>ASVHGTTYELLRRQGIDTVFGNPGSNELPFLKDFPEDFRYILALQEACVVGIADGYAQASRKPAFINLHSAAGTGNAMGALSNAWNSHSPLIVTAGQQTRAMIGVEALLTNVDAANLPRPLVKWSYEPASAAEVPHAMSRAIHMASMAPQGPVYLSVPYDDWDKDADPQSHHLFDRHVSSSVRLNDQDLDILVKALNSASNPAIVLGPDVDAANANADCVMLAERLKAPVWVAPSAPRCPFPTRHPCFRGLMPAGIAAISQLLEGHDVVLVIGAPVFRYHQYDPGQYLKPGTRLISVTCDPLEAARAPMGDA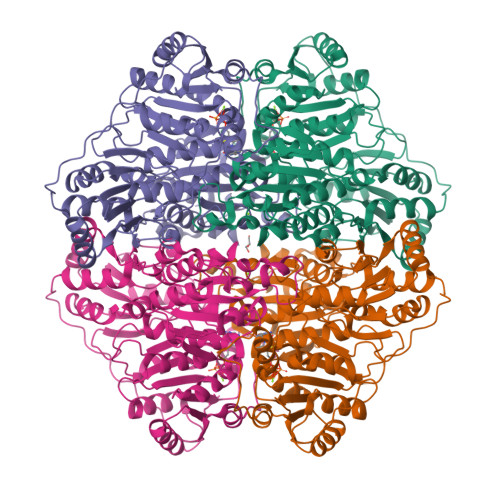IVADIGAMASALANLVEESSRQLPTAAPEPAKVDQDAGRLHPETVFDTLNDMAPENAIYLNESTSTTAQMWQRLNMRNPGSYYFCAAGGLGFALPAAIGVQLAEPERQVIAVIGDGSANYSISALWTAAQYNIPTIFVIMNNGTYGILRWFAGVLEAENVPGLDVPGIDFRALAKGYGVQALKADNLEQLKGSLQEALSAKGPVLIEVSTVSHHHHHH[4x]> GSHMASMKKKGSVVIVGRINLSGDTAYAQQTRGEEGCQETSQTGRDKNQVEGEVQIVSTATQTFLATSINGVLWTVYHGAGTRTIASPKGPVTQMYTNVDKDLVGWQAPQGSRSLTPCTCGSSDLYLVTRHADVIPVRRRGDSRGSLLSPRPISYLKGSAGGPLLCPAGHAVGIFRAAVSTRGVAKAVDFIPVESLETTMRSP

The HCV NS3/4A protease – a chymotrypsin-like serine protease – is a prime therapeutic target that cleaves four known sites along the virally encoded polyprotein. The NS3/4A protease also hydrolyzes two human proteins, TRIF and MAVS, which are part of the innate immune system, thereby confounding the innate immune response to viral infection. In this study, we report that four chemically representative protease inhibitors – telaprevir, danoprevir, vaniprevir and MK-5172 – exhibit distinct susceptibilities to the protease variants R155K, A156T and D168A. To elucidate the underlying mechanism by which chemically diverse inhibitors bind to the wild-type protease and drug-resistant variants, crystal structures were determined for 16 inhibitor-protease complexes. These complexes include wild-type protease and resistant variants R155K, D168A and A156T each bound to telaprevir, danoprevir, vaniprevir and MK-5172, with resolutions ranging from 1.10–2.50 Å; S139A protease variants were used except for telaprevir, which requires covalent bond formation with the serine 139 for efficient binding.

Against wild-type protease, macrocyclic inhibitors danoprevir, vaniprevir and MK-5172 exhibited antiviral potencies in the sub nM range (IC50 = 0.24, 0.34 and 0.11 nM, respectively), while telaprevir potency was significantly lower (IC50 = 1030 nM), consistent with previous reports. The acylsulfonamide groups of danoprevir, vaniprevir and MK-5172 were also positioned in the oxyanion hole, hydrogen bonding with the same set of backbone amide nitrogens, as observed previously for the TMC435 and danoprevir structures. Meanwhile the Nε nitrogen of H57 interacted with the sulfonamide nitrogen in these complexes, suggesting that the Nε atoms were deprotonated. In wild-type complexes involving macrocyclic inhibitors, R155 adopted a conformation distinct from those observed in telaprevir and substrate complexes to allow binding of the extended P2 moieties in the S2 subsite. This R155 conformation is stabilized by hydrogen bond interactions involving D168 and D80. Vaniprevir, with the P2 isoindoline moiety, bound in a conformation similar to danoprevir, making favorable cation-π stacking interactions with R155, despite the P2–P4 macrocycle.> MELSPTYQTERFTKFSDTLKEFKIEQNNEQNPIDPFNIIREFRSAAGQLALDLANSGDESNVISSKDWELEARFWHLVELLLVFRNADLDLDEMELHPYNSRGLFEKKLMQDNKQLYQIWIVMVWLKENTYVMERPKNVPTSKWLNSITSGGLKSCDLDFPLRENTNVLDVKDKEEDHIFFKYIYELILAGAIDEALEEAKL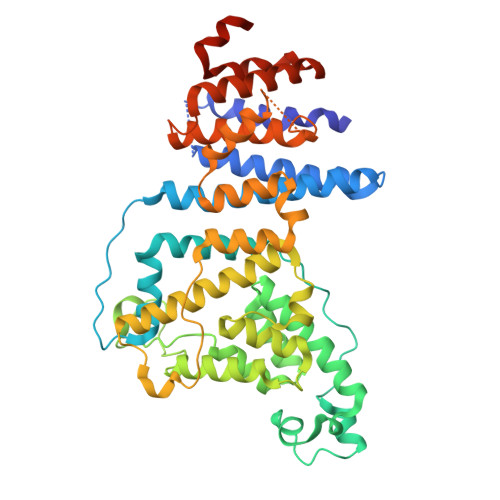SDNISICMILCGIQEYLNPVIDTQIANEFNTQQGIKKHSLWRRTVYSLSQQAGLDPYERAIYSYLSGAIPNQEVLQYSDWESDLHIHLNQILQTEIENYLLENNQVGTDELILPLPSHALTVQEVLNRVASRHPSESEHPIRVLMASVILDSLPSVIHSSVEMLLDVVKGTEASNDIIDKPYLLRIVTHLAICLDIINPGSVEEVDKSKLITTYISLLKLQGLYENIPIYATFLNESDCLEACSFILSSLEDPQVRKK4-[(2~{R})-butan-2-yl]phenol | 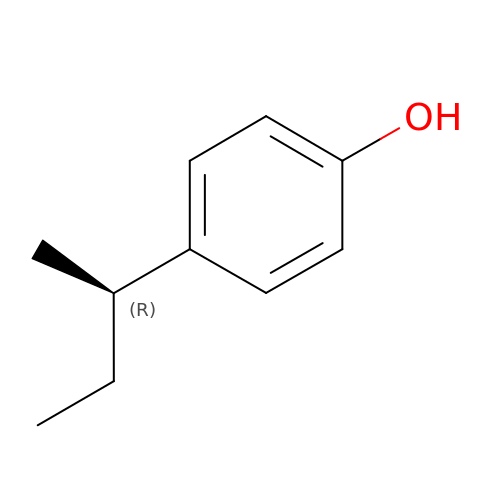C10 H14 O | ZUTYZAFDFLLILI-MRVPVSSYSA-N> SAKALIVYGSTTGN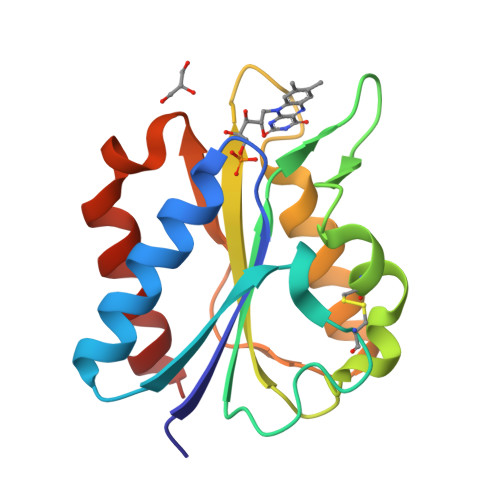TEYTAETIARELADAGYEVDSRDAASVECGGLFEGFDLVLLGCSTWGDDSIELQDDFIPCFDSLEETGAQGRKVACFGCGDSSWEYFCGAVDAIEEKLKNLGAEIVQDGLRIDGDPRAARDDIVGWAHDVRGAI> MSMLKREDWYDLTRTTNWTPKYVTENELFPEEMSGARGISMEAWEKYDEPYKITYPEYVSIQREKDSGAYSIKAALERDGFVDRADPGWVSTMQLHFGAIALEEYAASTAEARMARFAKAPGNRNMATFGMMDENRHGQIQLYFPYANVKRSRKWDWAHKAIHTNEWAAIAARSFFDDM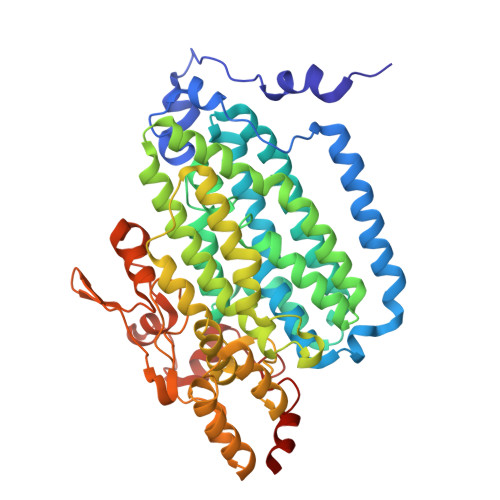MMTRDSVAVSIMLTFAFETGFTNMQFLGLAADAAEAGDHTFASLISSIQTDESRHAQQGGPSLKILVENGKKDEAQQMVDVAIWRSWKLFSVLTGPIMDYYTPLESRNQSFKEFMLEWIVAQFERQLLDLGLDKPWYWDQFMQDLDETHHGMHLGVWYWRPTVWWDPAAGVSPEEREWLEEKYPGWNDTWGQCWDVITDNLVNGKPELTVPETLPTICNMCNLPIAHTPGNKWNVKDYQLEYEGRLYHFGSEADRWCFQIDPERYKNHTNLVDRFLKGEIQPADLAGALMYMSLEPGVMGDDAHDYEWVKAYQKKTNAA>MDYMELAKEAFSIICTFIAAYVAYYYAIKQLHQKSVENIEYAKYQAVLQAHKSLYKLLRFTTNTENEDSILIWEKTKDGKQEATYYFRKENIRKFIKELSKEIYNEGCGIFMSKEALSLISEYRNIVYGFMLSAQNNPQETIRITNRESVERMKKIHQNLSIEIRQAINL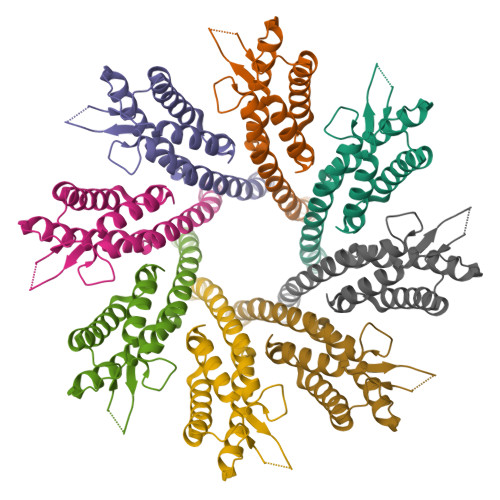KKRDLRFENLYFQ[8x]3-(2,3-dihydro-1,4-benzodioxin-6-yl)-5-(morpholin-4-yl)-7H-thieno[3,2-b]pyran-7-one | C19 H17 N O5 S | 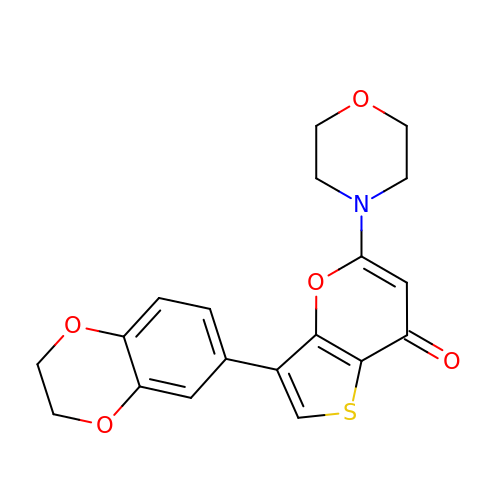BYTKNUOMWLJVNQ-UHFFFAOYSA-N> SNRPMPLNIYQFKNMIQCTVPSRSWWDFADYGCYCGRGGSGTPVDDLDRCCQVHDNCYNQAQEITGCRPKWKTYTYECSQGTLTCKGRNNACAATVCDCDRLAAICFAGAPYNDN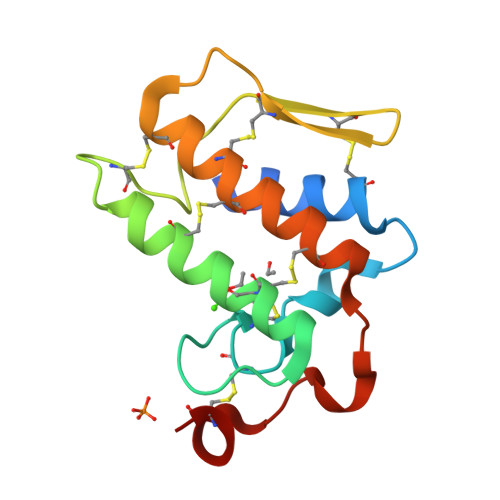NYNIDLKARCQ>MGSSHHHHHHSSENLYFQGHSKSPRKDYAKLANYDESKVPQYTLPSVLMCHDGEMVQTKEQWEQKRRPEILNLFTTYMFGKAPVLKHKLPCTVSRINEKALNGRATRKEITIQLTDDPQGPHIDLQLYLPNHVSGKIPVFLGISFMPNYTIYDDPDLSVPEITDEKMKKRSFRGSMDKSWQLDKILEHGYGLATFCYNDVDPDFDDDFQNGVHPYYYEKGQNFPDPDQWGSIAAWAWGMSRAMDYLETDKKVDAKKVAVIGHSRLGKTAVWAGASDPRFALVISGNSGCCGVAISRRCFGETVEAMNVRFPHWFCGNYKQFNDREKYLPFDQHELVALIAPRPIYIASAEEDNWSDQKGEFLGGKGAEPVYALYGLGGIGCEEMPPVDTPYMNGPIAYHNRKGPHAVLPYDWEQFLRFADKYFKNK[2x]

Glucuronoyl esterases from carbohydrate esterase family 15 (CE15) have been proposed as an aid in reducing this recalcitrance by cleaving ester bonds found between lignin and glucuronoxylan. Only PvCE15 proved amenable to crystallization, and its structure was solved both as an apo protein and in complex with GlcA and GalA, respectively. PvCE15 has an α-/β-hydrolase fold like previously determined CE15 structures, consisting of a three-layer sandwich with a solvent-exposed cleft comprising the active site. The catalytic triad (Asp353-His406-Ser264) and oxyanion-stabilizing arginine (Arg265, oxyanion hole), whose positions and roles have been established in previous work on CE15 GEs, are conserved in PvCE15.

Attempts to obtain a Michaelis complex with the substrate BnzGlcA were unsuccessful but afforded GlcA complexes in both protomers in the asymmetric unit with the ligand bound in the same orientation as other GE-GlcA complexes. A notable distinction from previously determined CE15 members is the presence of an arginine residue in PvCE15 found at the edge of the binding cleft whose side chain, found projecting away from the pocket in the native structure, is rotated inward with its guanidinium positioning the glucuronate O2. Conserved are also the highly conserved residues supporting glucuronate binding within CE15, such as the tryptophan, glutamate, and lysine residues found interacting with the glucuronate O2, O2 and O3, and O4 hydroxyls, respectively (Trp355, Glu302, and Lys268). Crystals of the apo and ligand-soaked structures were both of space group P21 and contained two molecules in the asymmetric unit with similar cell dimensions. We considered the possibility that these enzymes might bind GlcA and GalA in distinct ways which could then facilitate action upon backbone residues. To investigate this, we obtained crystal structures of PvCE15 in complexes with both ligands. Although observed to bind in different orientations, neither orientation could easily be envisioned to support uronic acid being part of a main chain with linkages at the O1 and O4 positions, as is the case in the galacturonan backbone.>MAEQVLPQALYLSNMRKAVKIRERTPEDIFKPTNGIIHHFKTMHRYTLEMF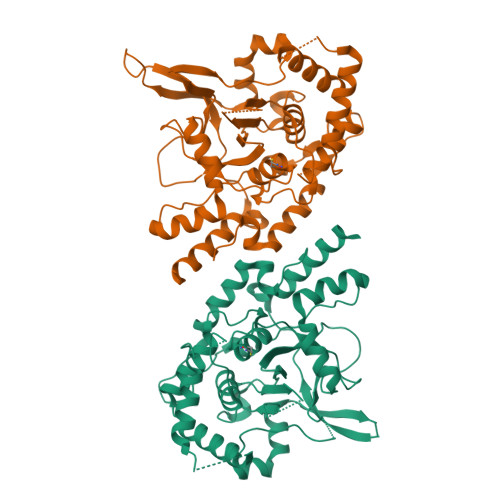RTCQFCPQFREIIHKALIDRNIQATLESQKKLNWCREVRKLVALKTNGDGNCLMHATSQYMWGVQDTDLVLRKALFSTLKETDTRNFKFRWQLESLKSQEFVETGLCYDTRNWNDEWDNLIKMASTDTPMARSGLQYNSLEEIHIFVLCNILRRPIIVISDKMLRSLESGSNFAPLKVGGIYLPLHWPAQECYRYPIVLGYDSHHFVPLVTLKDSGPEIRAVPLVNRDRGRFEDLKVHFLTDPENEMKEKLLKEYLMVIEIPVQGWDHGTTHLINAAKLDEANLPKEINLVDDYFELVQHEYKKWQENSEQGRRE[6x]Universal stress proteins (USP) are widely spread proteins in nature. In stress conditions such as heat shock, nutrient starvation, the presence of oxidants, uncouplers, DNA-damaging agents, or other stress agents which may arrest cell growth, USP constitute a natural biological defense mechanism. Under stress, USPs are overproduced and through a variety of mechanisms aid the organism in surviving in such uncomfortable conditions. Here, we present the structures of both apo- and cofactor-bound forms of an euryarchaeal USP AF0826 from A. fulgidus and a bacterial USP NE1028 from N. europaea.

The structure of the apo form of AF0826, a euryarchaeal USP from A. fulgidus was refined to a final resolution of 1.97 Å. The monomer structure is very similar to the structure of previously described NE1028 USP. In all other known USP structures, the residues found between strands β4 and β5 region form a loop. In contrast, the apo-AF0826 and AF1760-AMP structures were determined to contain chloride ions, which are not located in the same place as the divalent ions, while AF1760 still contains the ligand molecule. The chloride ions present in both structures may come from the crystallization solution or cell and play some other role if any. AF0826 displays the same type 1 dimerization, the dimerization interface is formed by β5 and α4 from each monomer as it takes place is case of NE1028.

>MGSSHHHHHHSSGRENLYFQGMIYMPIVVAVDKKSDRAERVLRFAAEEARLRGVPVYVVHSLPGGGRTKDEDIIEAKETLSWAVSIIRKEGAEGEEHLLVRGKEPPDDIVDFADEVDAIAIVIGIRKRSPTGKLIFGSVARDVILKANKPVICIK[4x]N~5~-[2-(propylsulfanyl)ethanimidoyl]-L-ornithine 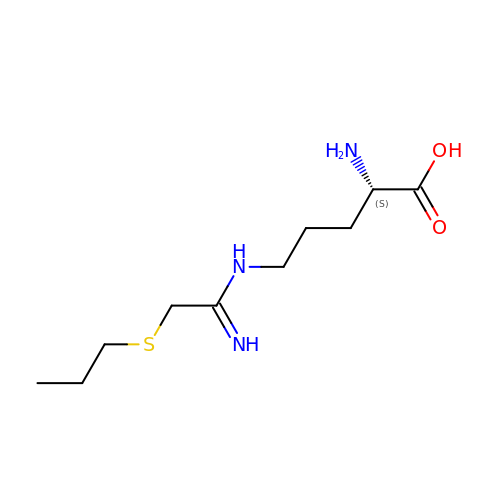| C10 H21 N3 O2 S | RLVQEZKGBMYDBZ-QMMMGPOBSA-N3-(9-HYDROXY-1,3-DIOXO-4-PHENYL-2,3-DIHYDROPYRROLO[3,4-C]CARBAZOL-6(1H)-YL)PROPANOIC 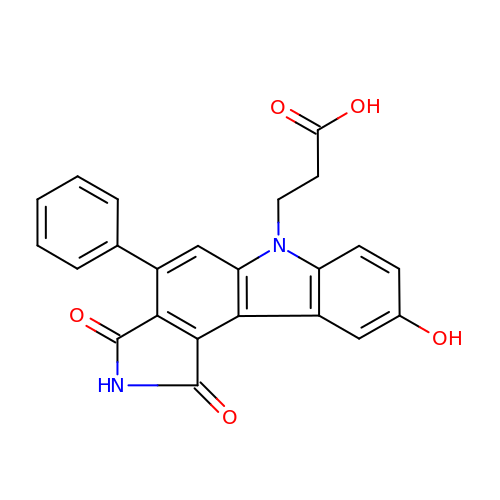ACID | C23 H16 N2 O5 | JDARUOOLJCFUOY-UHFFFAOYSA-N> MKNFKISSTYRAARKQQKTANRKSFY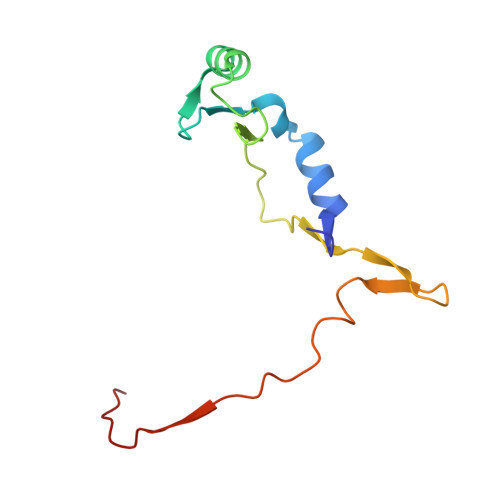NDEGYMISPSEWADGVIKGLINPKNSWSNDHVKGYLPRVSPRSHWTKNGYREYLGIGKSRDIPEKEPEVIEMMDLELVV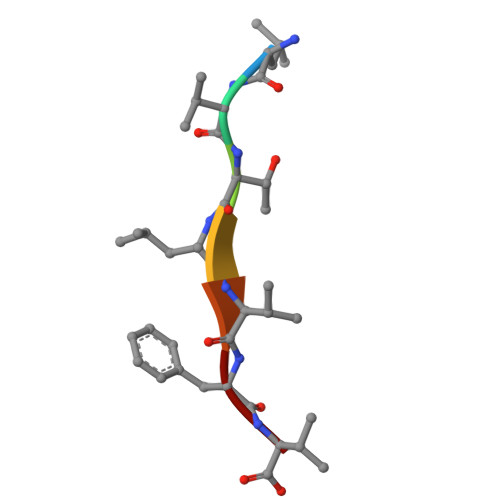> LVTLVFV> MESVADIQQLEEKVDESDVRIYFNEKSSGGKISIDNASYNARKLGLAPSSIDEKKIKELYGDNLTYE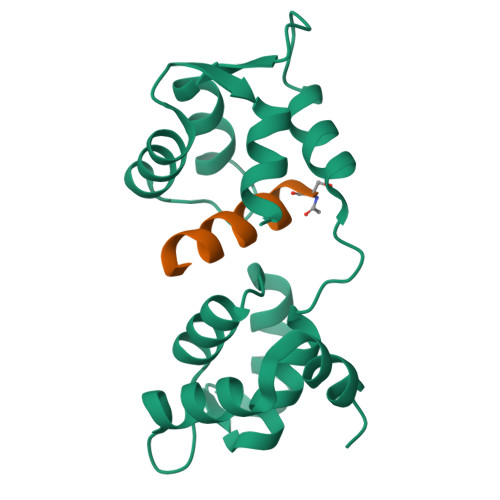QYLEYLSICVHDKDNVEELIKMFAHFDNNCTGYLTKSQMKNILTTWGDALTDQEAIDALNAFSSEDNIDYKLFCEDILQ;> SLMRVQAHIRKRMVA>MKFGIEFVPNEPIEKIVKLVKLAEDVGFEYAWITDHYNNKNVYETLALIAEGTETIKLGPGVTNPYVRSPAITASAIATLDELSNGRATLGIGPGDKATFDALGIEWVKPVSTIRDAIAMMRTLLAGEKTESGAQLMGVKAVQEKIPIYMGAQGPMMLKTAGEISDGALINASNPKDFEAAVPLIKEGAEAAGKSIADIDVAAYTCCSIDEDAAAAANAAKIVVAFIAAGSPPPVFERHGLPADTGKKFGELLGKGDFGGAIGAVDDALMEAFSVVG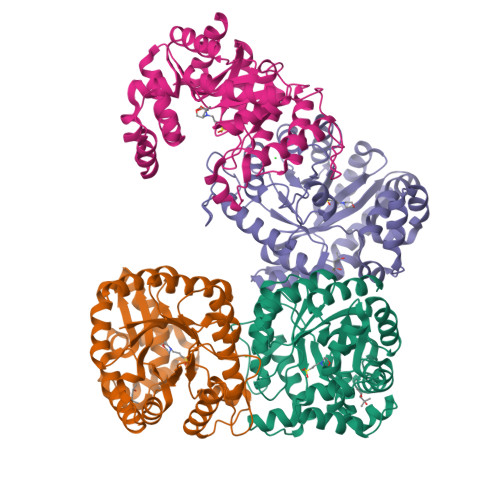TPDEFIPKIEALGEMGVTQYVAGSPIGPDKEKSIKLLGEVIASF[4x]2-[2-(4-oxocyclohexa-2,5-dien-1-ylidene)hydrazinyl]benzoic acid 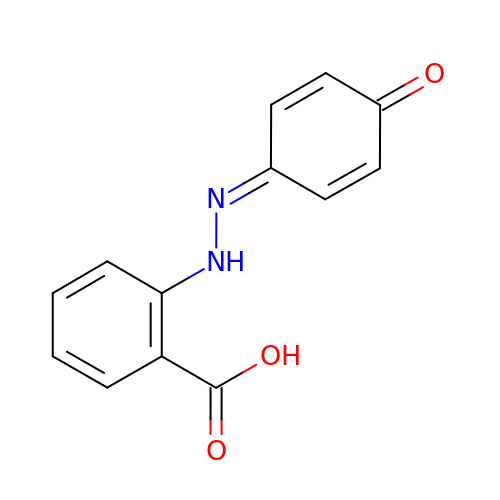| C13 H10 N2 O3 | FBVSMDPNVYJNON-UHFFFAOYSA-N> ETG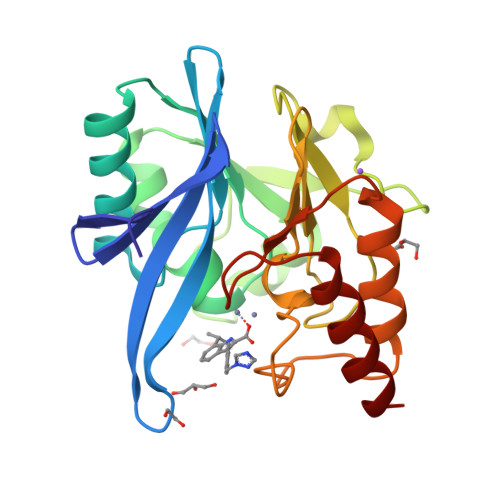DQRFGDLVFRQLAPNVWQHTSYLDMPGFGAVASNGLIVRDGGRVLVVDTAWTDDQTAQILNWIKQEINLPVALAVVTHAHQDKMGGMNALHAAGIATYANALSNQLAPQEGLVAAQHSLTFAANGWVEPATAPNFGPLKVFYPGPGHTSDNITVGIDGTDIAFGGCLIKDSKAKSLGNLGDADTEHYAASARAFGAAFPKASMIVMSHSAPDSRAAITHTARMADKLR> GGTIARTIVLQESIGKGRFGEVWRGKWRGEEVAVKIFSSREERSWFREAEIYQTVMLRHENILGFIAADNKDNGTWTQLWLVSDYHEHGSLFDYLNRYTVTVEGMIKLALSTASGLAHLHMEIVGTQGKPAI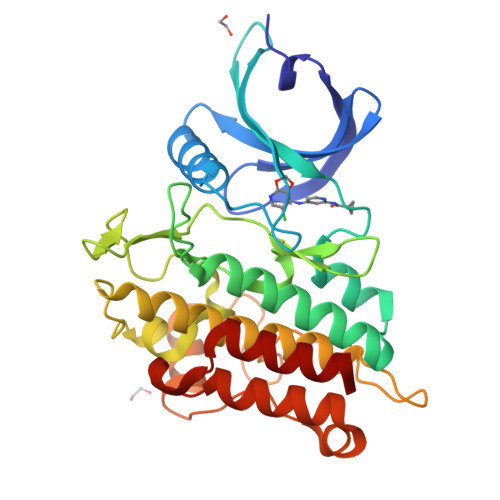AHRDLKSKNILVKKNGTCCIADLGLAVRHDSATDTIDIAPNHRVGTKRYMAPEVLDDSINMKHFESFKRADIYAMGLVFWEIARRCSIGGIHEDYQLPYYDLVPSDPSVEEMRKVVCEQKLRPNIPNRWQSCEALRVMAKIMRECWYANGAARLTALRIKKTLSQLSQQ> MPVVKGGVWTNIEDEILKAS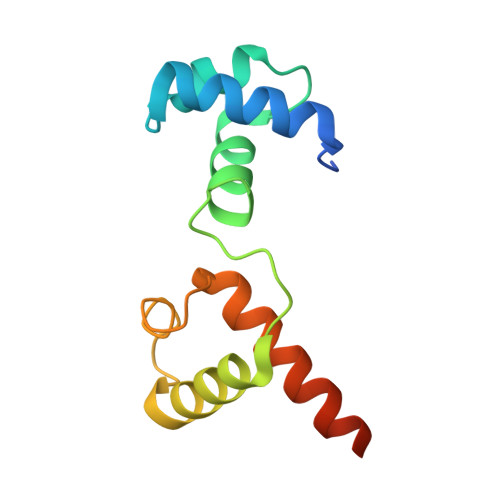VSKYGLNQWARVSSLLARKTPKQCKARWNEWLDPSIRKIEWSKDEDEKLLHLAKLMPTQWRTIAPIVGRTANQCLERYQKLLDEAEAALGHHHHHH>METKEIFDAAPLSVSQFLSETGQGLYIPPYQRAYSWELPKIRRLLSDVAHGLDQLAEFEDSICFLGTVIALRDINYTTVEPKYRSQVPSKVMTIIDGQQRMTTLLLLTTVLHEEIRVRAEKLTRDDEPSVWCYNQALDVTGRLSNCFEEDMRYGEHRYYPRLIRSYYDVWSRNKGEARYRSPIGYYLESYGAYARDPDAVKPYRHVPIDPDKTDGVDLEAYRHLDRMRDQMRSMLRKAVGAGVKREDDIQLPTGTDIGQSQNLQFALFNSEFPPSVVEQLEDDAKMTPLTRLIVFANYLLHRVTVAVVTAKREDYGFDMFEALNTTGQPLTAIETFKPRAIKEEGLDEWQESESKLHFDVVEAYLDREGSSSADKRQTVTSSVLLPFAMFQDGTKLTKRLNDQRRYLRTVFDKDPDIVARRKVLAGLAQVARFYEGPWGSPTKVPSCDDATLRTQAGIALAALREGGHDIVVGLLTRYFAAHRLSSPETVESSARQFLLAARSCAAFYALWRGSFGSTAGIDGVYRSLMTHVVEEGMPRFARFERDLTEVPPVEALQSYLKEQLRSEGIYDKQQWVARAAMTPVYQHSKPLTRLLLLAASQNSTPDSATPGLVVRGKSGLLETLELERWNDEAFATIEHVAPQAPSSNGSWNADLYEDPELINR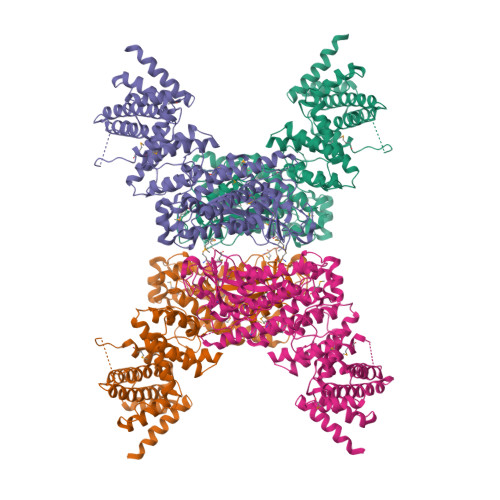IGNLTLLPAVENASASNRAWHLKRLMFRALSAATVEEAEKTLADAEAQGLRLGSGAGEIVRQARYLPLVAALAQREEEWTAEFVEARSQRLCSLAWDALTPWLGFEP[4x]> EVDKRREINNEHPLLMMPLYANGEEFNQGKYTFWGGDTLTGKWENIPDDLKPYTVIQLHPDDLPKRDGAARDFYEHMLEEAAKYVNPKTGKNEPIPVILTVYTAGNMPYHTSAHWLSTSWIDKMYQKYPNLHGIFSTESYWIWANDIENKAADYLKVSAKNGGYFIWAEQNSGSAIEKAFGKNGKIAFQKSVDKYWKNLIFMFKNTPAAEGNDSTTESYMKGLWLSNHTYQWGGLMDTWKWYETGKWKLFASGNIGKSQGDRQWLTEPESMLGEEALGVYLNGGVVYNFEHPAYTYGVNNKESLLFSEVIKEFFRYVIAHPAPSKEKVLEDTKVFIHGDYSNKGNGKFFVNVNTDREQTPLYMTGRYNVIPAIPGVLKTDKLKESVSSSRIQIKEITSPEFSSTQARKEYLNKLYPMNYEGDIFAQKLDNRWFVYNYKVNENVKQTG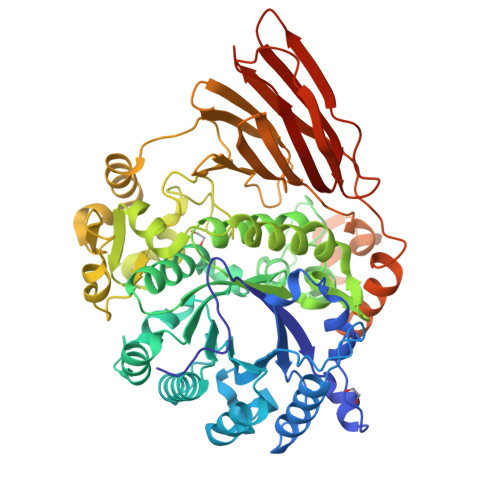KLKFNSLEMNVEFEPHTYGIFERISNGLKVNLNNFRTNKDSLWSNAQDANQAKKLPQLTKKGAIKWIEEHYIKDTQFGEKRVTKIVLRGIDKLPTIHSLSGTNNSYDQPSLNFDQKNHMVTITINSNGNLEFELHFLEHTRAPPPPPLRSGC Bacteriophage PR772 is a ﻿double-stranded DNA (dsDNA) virus with a 70 nm diameter icosahedral protein capsid encapsulating the internal lipid bilayer along with numerous proteins and a 15 kbp long linear genome. It belongs to the Tectiviridae family and infects gram negative hosts like Escherichia coli, ﻿Salmonella typhimurium and other bacteria, carrying a R772 plasmid-encoded receptor complex through which DNA can be transported during bacterial conjugation. In previous studies on PRD1, it was shown that the capsid is formed by proteins P3 (major capsid protein), P30 (capsid associated protein) and the vertex complex. The vertex complex includes the penton protein (P31), the host-recognition protein (P5) and the receptor-binding protein (P2) along with the infectivity protein (P16) that acts as a cementing protein, holding the vertex complex together and also stabilizing the pseudo-icosahedral capsid of the virus.

The structure of bacteriophage PR772 was determined by electron cryo-microscopy. The overall resolution determined by Fourier shell correlation (FSC) @0.143 was 2.75 Å. The resolution in most of the regions was high enough (3.2 Å – 2.3 Å) to build a de-novo model of the asymmetric unit comprising of P3, P30, P5, P31 and P16 into the icosahedrally averaged CryoEM map. The CryoEM 3D reconstruction of PR772 shows that the viral particle follows a pseudo T = 25 lattice architecture with a (h,k) of resulting in an icosahedral structure with 20 large trisymmetrons and 12 penta-symmetrons. The P3 monomers (subunits a, b and c) are interlocked to form a trimer that appears as a hexon. The high-resolution structure of PR772 confirms the previously shown variability of the N and C-terminals of the P3 protein depending on the locations within the trisymmetron. The high-resolution also allows us to extend the analysis of these conformations and show that the N-terminal of P3 can adopt three different conformations, not two as previously described. The newly discovered conformation of the N-terminal region of P3, a long helix with a kink, is structurally critical to accommodate the interlocking region formed by the N-terminal hooks of P30 during the initiation of particle assembly. P30 adopts an extended conformation in an intact viral particle and it is found wedged in between the trisymmetrons. Five copies of P16 bridge the penton to the five trisymmetrons that meet at the vertex complex. Our studies show that unlike what was predicted for PRD1, the penton base of PR772 is an asymmetric heteropentamer consisting of three copies of P5 and two copies of P31.

>[12x]MAQVQQLTPAQQAALRNQQAMAANLQARQIVLQQSYPVIQQVETQTFDPANRSVFDVTPANVGIVKGFLVKVTAAIKNNHATEAVALTDFGPANLVQRVIYYDPDNQRHTETSGWHLHFVNTAKQGAPFLSSMVTDSPIKYGDVMNVIDAPATIAAGATGELTMYYWVPLAYSETDLTGAVLANVPQSKQRLKLEFANNNTAFAAVGANPLEAIYQGAGAADCEFEEISYTVYQSYLDQLPVGQNGYILPLIDLSTLYNLENSAQAGLTPNVDFVVQYANLYRYLSTIAVFDNGGSFNAGTDINYLSQRTANFSDTRKLDPKTWAAQTRRRIATDFPKGVYYCDNRDKPIYTLQYGNVGFVVNPKTVNQNARLLMGYEYFTSRTELVNAGTISTT;> MALINPQFPYAGPVPIPGPAPTETMPLLNYRVEGRIAGIQQARQFMPFLQGPHREVAEQTYYAIGTGIQMGQTFNQPLINTQEG;> MDKKKLLYWVGGGLVLIIIWLWFRNRPAAQVASNWEGPPYMTYNQPQAGSVTLPVAGYTSPSLTLPNRNRSCGCNPAVSAAMAQGADLASKLTESISSQLNNYAESLNDYLASQAGV;>[3x]MANQQIGGSTVTYNGAIPMGGPVAINSVIEIAGTEVLVDLKLDYATGKISGVQTLYIDLRDFLGDVTVTMPDTGQRITARAGTQGYYPVLSTNLMKFIVSATIDGKFPMNFINFPIALGVWPSGIKGDKGDPGAPGPAGGTVVVEDSGASFGESLLDTTSEPGKILVKRISGGSGITVTDYGDEVEIEASGGGGGGGGVTDALSLMYSTSTGGPASIAANALTDFDLSGALTVNTVGTGLTKSAAGIQLAAGKSGLYQITMTVKNNTVTTGNYLLRVKYGSSDFVVACPASSLTAGGTISLLIYCDVLGVPSLDVLKFSLCNDGAALSNYIINITAAKIN;>MNVNNPNQMTVTPVYNGCDSGEGPQSVRGYFDAVAGENVKYDLTYLADTQGFTGVQCIYIDNAENDGAFEIDVEETGQRIKCPAGKQGYFPLLVPGRAKFVARHLGSGKKSVPLFFLNFTIAQGVW[2x]>GHVPRIAEVRDAAEPSSEEQRARHVRMLEAAIELATEKELARVQMHEVAKRAGVAIGTLYRYFPSKTHLFVAVMVDQIDRMGVGFKKSAPPGESPQDAVYNVLVRATRGLLRRPALSTAMIQSTSTANVASVPDAGKVDRAFRQIMLDAAGIEHPTEEDLTALRLLVQLWFGVIQSCLNGRVSIPDAESDIRRA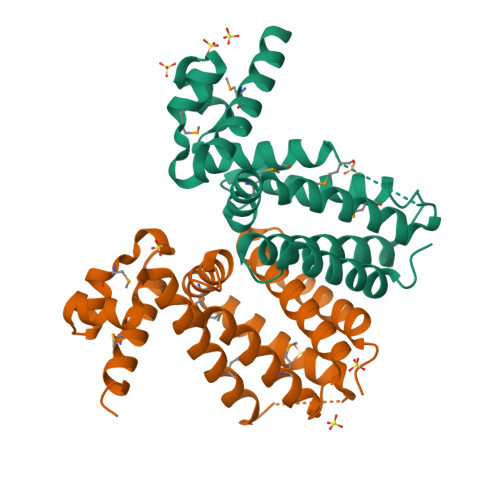CDLLLVNLSHRGS[6x]> SNAMSDSLRIIFAGTPDFAARHLGALLSSQHKIVGVFTQPDRPAGRGNKLTPSPVKILAEHHGIPVFQPKSLRPEENQHLVADLNADIMVVVAYGLILPAAVLAMPRLGCINVHGSLLPRWRGAAPIQRSVWAGDEKTGITIMQMDIGLDTGAMLHKIECAIQPEDTSATLYDKLAQLGPQGLLITLQQLAAGTALAEVQNETQATYAEKLSKEEAKLDWTLSATQLERCIRAFNPWPVSYFIVDEQPIKVWQAQVLPAGEDAEPGTIIHADKHGIQVATADGV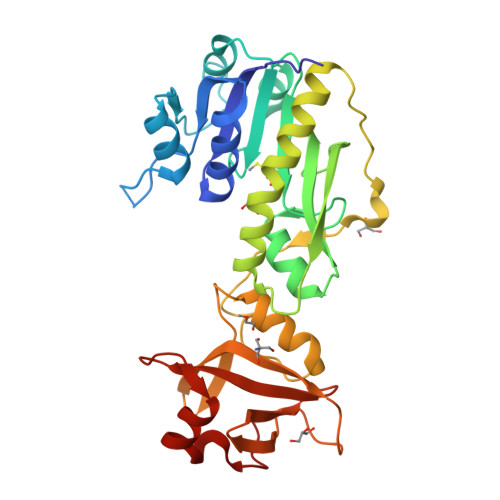LNITQLQPAGKKAMSAADLLNSRREWFIPGSQLV> PTLWPQREALKSALQYPALAGPVFDALTVEGFTHPEYAAVRAAIDTAGGTSA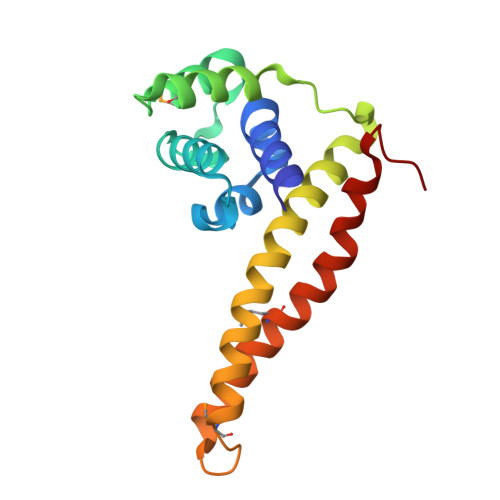GLSGAQWLDMVRQQTTSTVTSALISELGVEAIQVDDDKLPRYIAGVLARLQEVWLGRQIAEVKSKLQRMSPIEQGDEYHALFGDLVAMEAYRRSLLEQASGDDLHHHHHH We present the first atomic-resolution crystal structure of a multimeric ring form of a viral dsDNA packaging motor, the ATPase of the asccφ28 phage, and characterize its atomic-level dynamics via long timescale molecular dynamics simulations. In contrast, a close homolog of the φ29 ATPase from the related bacteriophage asccφ28 (gp11) has been shown to form highly soluble functional rings; extensive analytical ultracentrifugation and small-angle X-ray scattering experiments show that the ATPase forms pentameric rings in solution. Individual subunits within the ring are organized into two globular domains connected by a linker domain, each of which is nearly identical to the corresponding domains of the φ29 gp16. Like φ29 gp16, the N-terminal domain adopts the canonical ASCE ATPase fold, while the C-terminal domain is a ‘vestigial nuclease domain’.

Two crystal forms of gp11 were obtained: (i) tetragonal crystals belonging to space group P43212 and (ii) trigonal crystals belonging to space group P3221. While the three structures described here were determined in the absence of nucleotide, the active sites of ASCE ATPases are well characterized and can be accurately identified. Two distinct conformations of the Walker A motif are apparent in our crystal structures. One conformation binds either a SO42− or PO43− ion in the canonical β-phosphate position. The ion forms hydrogen bonds with the backbone of the Walker A motif in lieu of a β-phosphate, typically provided by ATP or ADP, which explains why the Walker A backbone adopts a conformation similar to a typical nucleotide-bound ATPase configuration. However, because the structure was solved in absence of nucleotide or nucleotide analog, it lacks any interactions mediated by the α- and γ-phosphates, ribose sugar, or adenosine base. Thus, this structure likely represents a conformation with mixed characteristics from both the apo and nucleotide-bound configurations. However, the crystal structure of asccφ28 gp11 ring reported here shows no such helicity in the N- or C-terminal domains. We suspect that we do not observe helicity in the crystal structures due to lack of substrate DNA imparting helicity.

>[5x]MITKSNEFWTPKRLLETDDRIFLVVGGRGVGKTFNVTGEALDDLFFNNVSMVYLRRLGVEIDELEKNNFITEEMLRVYFGNRFSDFNADESKQIMRFSIDGAIHEIKAIRNKIFFDDRCIVYFIALSRAGHVKSNNYPDVKYLVFDEVIIDRSIMPNARYIRNEFTVLLNLIETIKRKREDFYLFMLSNVGENFNPIFAGLGYYLTHEDIKKGFVKREDYCVQFVENKQEELNMTDPFVRLGAKNRDFSNSKTNAFENIRTPYFKHYGKKPKLLVKYDRQYLGIAERKIPSGLEYYYQVYKTLDGLENITVFNNNFDTLMEDEVFLEETQLKKKFKTYFELFQQNMVYHESPETFLEWSKFVYALKLEHHHHHH>GPLGSMATTNDSAVLFYIVASQKKLSFDY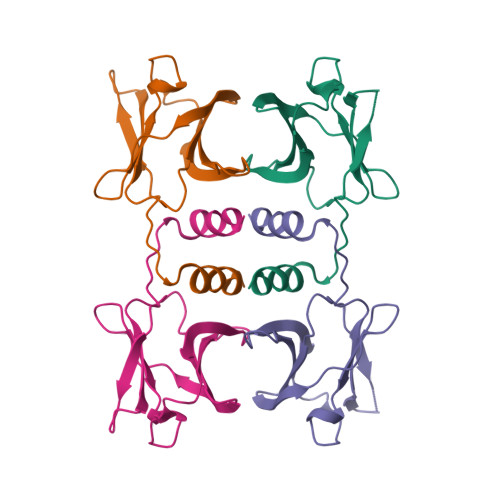TPNWGRGSPNSYIDALTFPRVLTNKPYKYRVVKAGQDLGVRDSYSVQSDGSQKVNFLEYNAGRGIADTQTIQVYVVDPDNGNQYLVAQWKHHHHHH[4x]> GPMADIGSNLQEDSLMKTQAELLLERLQEVGK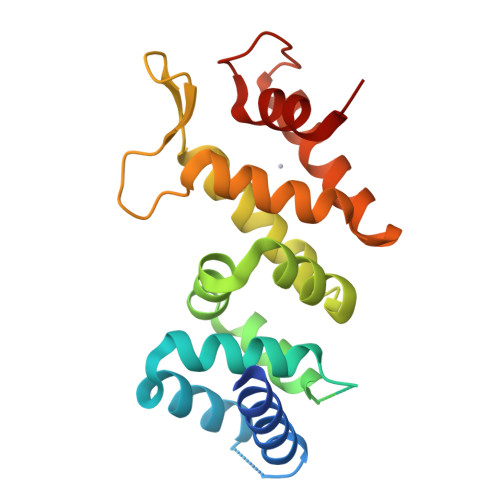AEAERPARFLSSLWERLPQNNFLKVIAVALLQPPLSRRPQEELEPGIHKSPGEGSQVLVHWLLGNSEVFAAFCRALPAGLLTLVTSRHPALSPVYLGLLTDWGQRLHYDLQKGIWVGTESQDVPWEELHNRFQSLCQAPPPLKDKVLTALETCKAQDGDFEVPGLSIWTDLLLALRSG6-(ethylamino)-2-(methylamino)-3,7-dihydro-8H-imidazo[4,5-g]quinazolin-8-one 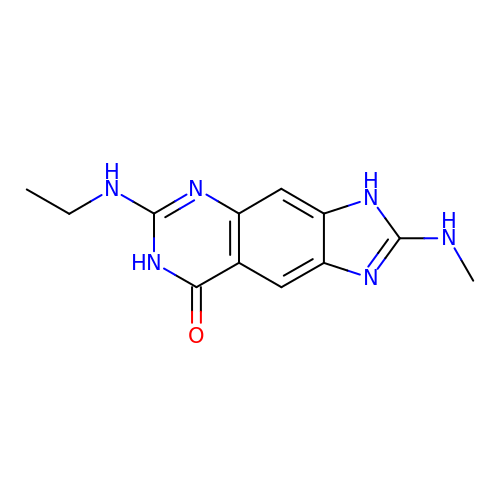| C12 H14 N6 O | SJNDGKATIKMROA-UHFFFAOYSA-N>MTQFNPVDHPHRRYNPLTGQWILVSPHRAKRPWQGAQETPAKQVLPAHDPDCFLCAGNVRVTGDKNPDYTGTYVFTNDFAALMSDTPDAPESHDPLMRCQSARGTSRVICFSPDHSKTLPELSVAALTEIVKTWQEQTAELGKTYPWVQVFEN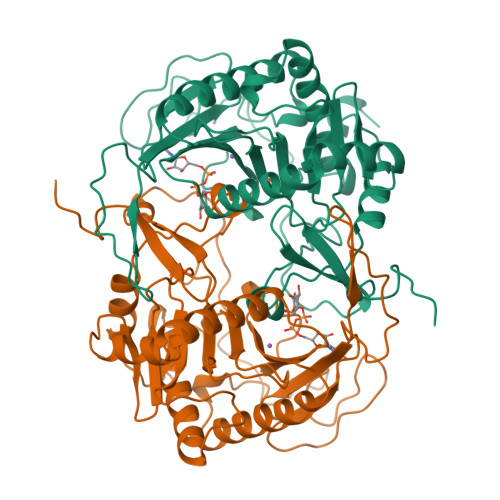KGAAMGCSNPHPGGQIWANSFLPNEAEREDRLQKEYFAEQKSPMLVDYVQRELADGSRTVVETEHWLAVVPYWAAWPFETLLLPKAHVLRITDLTDAQRSDLALALKKLTSRYDNLFQCSFPYSMGWHGAPFNGEENQHWQLHAHFYPPLLRSATVRKFMVGYEMLAETQRDLTAEQAAERLRAVSDIHFRESGV[4x]>[4x]M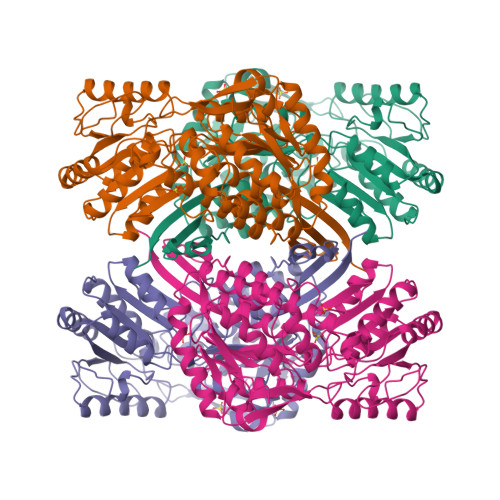TKQYKNYVNGEWKLSENEIKIYEPASGAELGSVPAMSTEEVDYVYASAKKAQPAWRALSYIERAAYLHKVADILMRDKEKIGAILSKEVAKGYKSAVSEVVRTAEIINYAAEEGLRMEGEVLEGGSFEAASKKKIAVVRREPVGLVLAISPFNYPVNLAGSKIAPALIAGNVIAFKPPTQGSISGLLLAEAFAEAGLPAGVFNTITGRGSEIGDYIVEHQAVNFINFTGSTGIGERIGKMAGMRPIMLELGGKDSAIVLEDADLELTAKNIIAGAFGYSGQRCTAVKRVLVMESVADELVEKIREKVLALTIGNPEDDADITPLIDTKSADYVEGLINDANDKGATALTEIKREGNLICPILFDKVTTDMRLAWEEPFGPVLPIIRVTSVEEAIEISNKSEYGLQASIFTNDFPRAFGIAEQLEVGTVHINNKTQRGTDNFPFLGAKKSGAGIQGVKYSIEAMTTVKSVVFDIK>[2x]MFKTEFEFPEELKTKLQEHINYFPKKRQAILLCLHEIQNYYGYIPPESLKPLADMLELPLNHVEGVVAFYDMFDREDKAKYRIRVCVSIVCHLMGTNKLLKALENILGIKPGEVTPDGKFKIVPVQCLGACSEAPVFMVNDDEYKFESEVQLNEILSRYT;>MRSYPAIPRIYAETTLNMLLKRAKKPRVHSIDEYLKDGGYQALEKALNMSPEEIIDWVDKSTLRGRGGAGFPTGKKWKFAVQNPGPRYFICNADEMEPGTFKDRIIIERDPHLLIEGIIISSYAIGANEAYIYIRGEYPAGYYILRDAIEEAKKKGFLGKNILGSGFDLEIYVARGAGAYICGEETALIESLEGKRGHPRLKPPYPVQKGLWGKPTVVNNVETIANVPFIISMGWEEYRYIGPSDYAGPKLFPVSGKVKKPGVYELPMNTTLREVIFKYAGGTLGNKKVKAVFSGALDCFSSEELDIPMDYSPLGFGGTGTVIVLTEEDDIVEAALKIAEFYEHETCGQCTPCRVGCYEQANLLEKIYKGEATEQDWEGFDFVNRNIQPTSICGLGAVAGRLIRQTLEKFPEEWEKYRKKSASLPLAGHHHHHH[2x]

Complex I couples the transfer of two electrons from NADH to ubiquinone (Q) with the translocation of four protons across the membrane. The L-shaped complex is structured into a peripheral arm that protrudes into the aqueous milieu and catalyzes electron transfer with one FMN and 8–10 iron–sulfur ([Fe–S]) clusters, and a membrane arm embedded in the lipid bilayer that mediates proton translocation. We have determined structures of the electron-input module of complex I from the hyperthermophilic bacterium Aquifex aeolicus, encompassing subunits NuoE and NuoF that contain the FMN cofactor, the [4Fe–4S] cluster N3, and the [2Fe–2S] cluster N1a, respectively, both in the air-oxidized and dithionite-reduced states at resolutions up to 1.8 Å. Here, we show that the redox state of N1a regulates NADH oxidation in complex I by inducing a conformational change close to the NADH-binding site.

To ensure that the methionine residue at the homologous position in the E. coli complex does not change the local structure, we generated, purified, and crystallized the A. aeolicus S96MF variant. The mutation did not impose any substantial structural changes, although the hydroxyl group of the original S96 is no longer available for hydrogen bonding to the peptide carbonyl of D94. In addition, the larger side chain of the methionine residue displaces two water molecules, while another water molecule shows up in a different position.>[2x]GENGESVVVLDKYGYPILYAPEEIGEEKEYSKYEDVVIEWNPSVTPVQIEKNYEVKFDVRQVKLRPPKVKNGSGKEGEIIVEAYASLFKSRLSKLKRILRENPEISNVVDIGKLNYVSGDEEVTIIGLVNSKRETNRGLIFEVEDKTGIVKVFLPKDSEDYREAFKVLPDAVVAFKGFYSKKGIFFANKFYLPDVPLYRKQKPPLEEKVYAILISDIHVGSREFCEKAFLKFLEWLNGHVESKEEEEIVSRVKYLIIAGDVVDGIGIYPGQYSDLVIPDIFDQYEALANLLANVPEHITMFIGPGNADAARPAIPQPEFYKEYAKPIYKLKNAIIISNPAVIRLHGRDFLIAHGRGIEDVVSFVPGLTHHKPGLPMVELLKMRHLAPTFGGKVPIAPDPEDLLVIEEVPDLVQMGHVHVYDAVVYRGVQLVNSATWQAQTEFQKMVNIVPTPAKVPVVDVESARVVKVLDFSGWC

PolD is an unusual archaeal replicative DNA polymerase (DNAP) in that it has all the functional properties of a replicative DNAP but with a catalytic core reminiscent of an RNA polymerase (RNAP). PolD is a heterodimeric replicative DNAP composed of a large catalytic subunit (DP2) and a smaller subunit with 3′-5′ proofreading exonuclease activity (DP1). A characteristic of PolD is that the exonuclease and polymerase active sites are hosted by two distinct subunits. Indeed, PolD has been shown to share an unexpected structural homology with the “two-double-psi β-barrel” (DPBB) family of RNAPs, which includes multisubunit transcriptases from all domains of life, homodimeric RNA silencing pathway RNAPs, and atypical RNAPs encoded by some viruses.

In order to prevent DNA degradation during cryo-EM preparation, the exonuclease-deficient variant PolD (DP1 H451A) was used in this experiment. The structure of the DP1 H451A (144–619) individual subunit was solved separately using X-ray crystallography at 2.6-Å resolution, ensuring that neither the overall structure of DP1 nor its two metal ion–binding sites are altered by the H451A mutation. All the density accounting for DP1 could be conveniently interpreted by rigid-body fitting the DP1 H451A individual crystal structure, with the DP1 EM and crystal structures showing only little differences. DP1 shows an oligonucleotide binding (OB) domain that is inserted within the N-terminal region of a large Mre11-like nuclease phosphodiesterase domain (PDE) whose active site entry faces the 3′ end of the nascent DNA strand. Second, the Mre11-like DP1 nuclease differs from the DnaQ-like exonuclease domains found in most DNAPs showing proofreading activity. Indeed, PDE domains are encountered in a wide range of hydrolases, but their dedication to DNAP-associated proofreading is specific to PolD.> MGSYIEREIKLRVISPSLEEIEERIRNNYTFINEEHQIDIYYNNPIRDFRKSDEA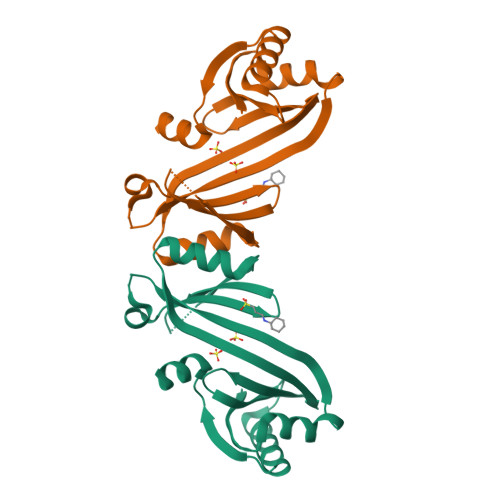LRLRNTNGKVILTYKGPKQSKETKTREEIEVEVSDLHKMDLILRKLGFIRSFQVEKIRKNYKYADFIISLDSIKELGEFIEIEGINKTEKELISFVDEFVKKHQIQYEKTIKSYLELLVEHAKKTNNSNTHGSIEGRHHHHHH>UUUGCUGAGGUGCACACAGCAAU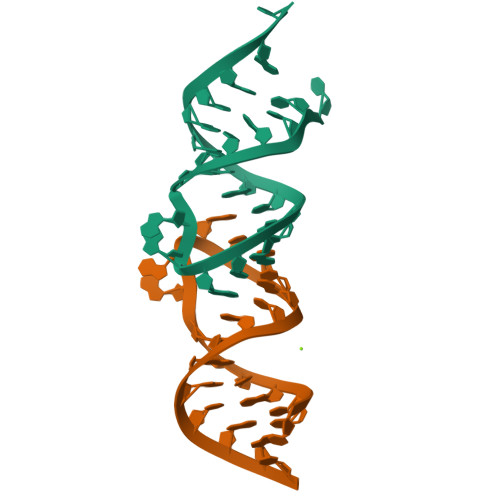[4x]N-(pyridin-4-ylmethyl)-2,3-dihydro-1,4-benzodioxin-6-amine 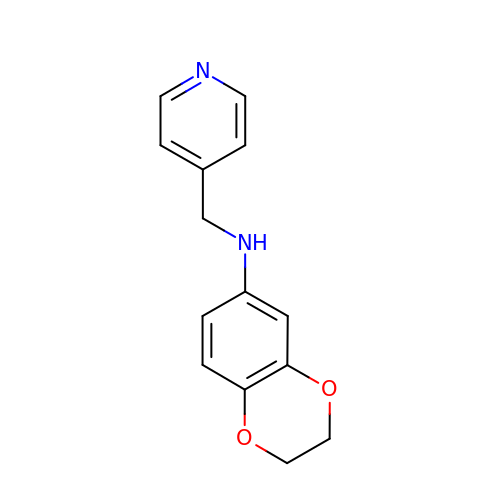| C14 H14 N2 O2 | ZEHRBOVXNPCYAK-UHFFFAOYSA-N2-fluoranyl-3-[6-(4-fluoranyl-3-oxidanyl-phenoxy)pyridin-2-yl]phenol 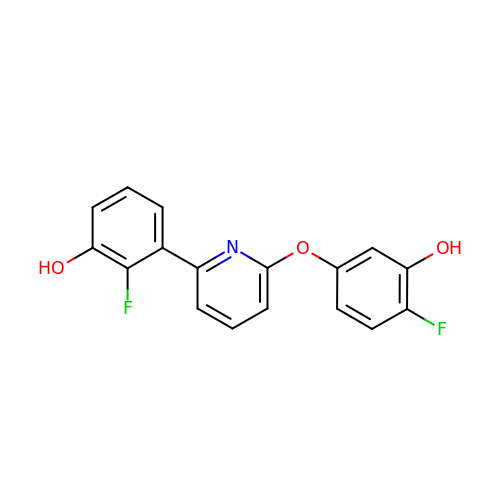| C17 H11 F2 N O3 | URNXTVXZHNOBRL-UHFFFAOYSA-N> HMASMTGGQQMGRGSDFGDIEERGKILVSLMYSTQQGGLIVGIIRCVHLAAMDANGYSDPFVKLWLKPDMGKKAKHKTQIKKKTLNPEFNEEFFYDIKHSDLAKKSLDISVWDYDIGKSNDYIGGCQLGI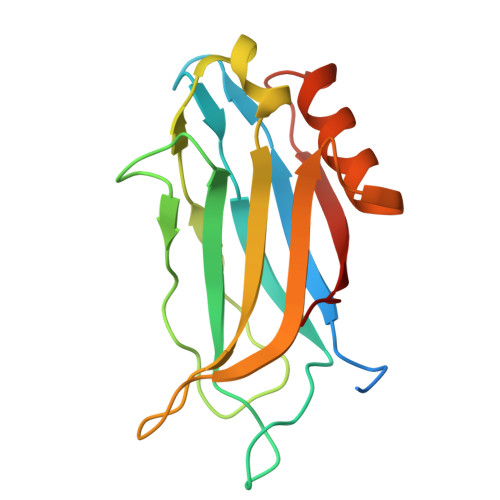SAKGERLKHWYECLKNKDKKIERWHQLQNENH>[4x]SSPADSYNEGVKPWRLQPQEISPPPTANLDRSNDKVYENVTGLVK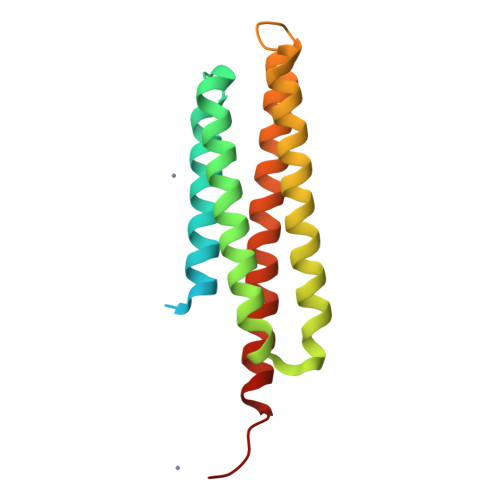AVIEMSSKIQPAPPEEYVPMVKEVGLALRTLLATVDETIPLLPASTHREIEMAQKLLNSDLGELINKMKLAQQYVMTSLQQEYKKQMLTAAHALAVDAKNLLDVIDQARLKMLGQTRPH> SNASVERVYQKKTQLEHILLRPDTYIGSVEPLTQFMWVYDEDVGMNCREVTFVPGLYKIFDEILVNAADNKQRDKNMTCIKVSIDPESNIISIWNNGKGIPVVEHKVEKVYVPALIFGQLLTSSNYDDDEKKVTGGRNGYGAKLCNIFSTKFTVETACKEYKHSFKQTWMNNMMKTSEAKIKHFDGEDYTCITFQPDLSKFKMEKLDKDIVALMTRRAYDLAGSCRGVKVMFNGKKLPVNGFRSYVDLYVKDKLDETGVALKVIHELANERWDVCLTLSEKGFQQISFVNSIATTKGGRHVDYVVDQVVGKLIEVVKKKNKAGVSVKPFQVKNHIWVFINCLIENPTFDSQTKENMTLQPKSFGSKCQLSEKFFKAASNCGIVESILNWVKFKAQTQLNKKCS

Human topoisomerase II beta (TOP2B) modulates DNA topology using energy from ATP hydrolysis. The N-terminal half of the ATPase domain contains the ATP-binding site and is directly involved in clamp closure, undergoing dimerization upon ATP binding. The C-terminal half of the ATPase domain forms the transducer domain, which connects the ATPase domain to the enzyme core (Oestergaard et al., 2004). A heart-shaped dimer is formed with a central cavity that is 31 Å high and 23 Å wide, the dimensions of which cannot easily accommodate a DNA duplex. Each TOP2B ATPase protomer folds into two discrete structural modules: the N-terminal GHKL domain and the C-terminal transducer domain (colored yellow and orange respectively in Figure 2A).

The structure was solved to 2.6 Å by molecular replacement using the TOP2B:AMPPNP structure as a search model. The final ADP-bound model contains residues 47–422 with missing loops between residues 169 and 173 and 356 and 366, where the K loop resides. The ADP structure is composed of a virtually unchanged GHKL domain compared with the AMPPNP structure, with the nucleotide and most of the active-site residues in the same conformation. The adenine ring, ribose sugar, and α phosphate of ADP make the same set of residue contacts as in the AMPPNP complex, despite the sugar pucker differing. As the γ phosphate is lost during ATP hydrolysis, R178 and N179, which were previously bound to the γ phosphate of AMPPNP, instead bind to the β phosphate of ADP. The γ phosphate-binding site is now occupied by a sulfate ion present in the crystallization condition (0.2 M ammonium sulfate), as is observed in TOP2A (Wei et al., 2005; Stanger et al., 2014). Thus, our ADP structure represents the post-hydrolysis state with the sulfate group mimicking the ATP hydrolysis product, Pi. The transducer domain of the ADP monomer opens up toward the C terminus of the protein (represented by dashed box in 4A), signifying the relaxed conformation. Moreover, during the reorganization of the transducer domain, the QTK loop is shifted away from the ATP-binding site (represented by dashed box in Figures 4B), preventing Q392 and K394 from making contacts with the nucleotide. Specifically, the side chain of Q392 moves by 3.8 Å and K394 moves by 2.5 Å.>MQKTLEVWIMPNSPQPAEDFKALVAPFEKAHGVEVKVTVLDWGVAWTKITTAATSGVGPDLTQLGTTAVGAISAMGVLEPVDDVLEALGGEKAYLPAVWRTTRLEGARQATAVPWFSELRAFYYRTDALKAAGVNPAEMFASWQGFEAGLARLKASSFRDPETKAPLAPLCTPGKNSWDVLHNAAPWIWGAGGEIVRQAGGRWQSALNSPESLEGLYFFLSLAQKGYVPAESLEKNTAQIEADFQAGKCAVFASGPWMIQRAQVPEAKGGFAERTAAKNLGVAPYPAGPKGRYTFFGGSNLALFNFSKNKPLAKELLKYLGGPEAQVRYAQMTGMLPALRSAWSDPSFQQNPLLRTFIQAAQFGRTYPSLAGWGGVENLAVQHLGMAWDL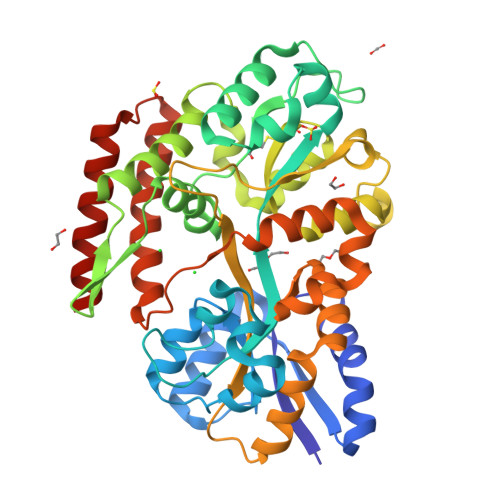VAQGRLTREALKDLMDKASAAINQALRHHHHHH[2x]>SNAMATNLIGLDTTQSQKLANALNNLLANYQVFYMNTRGYHWNIQGKEFFELHAKFEEIYTDLQLKIDELAERILTLSARPMHSFSGYLKAAQIKEHTDSIDGRSSMQGLVDGFSILLHQQRDILELAGETGDEGTSALMSDYIREQ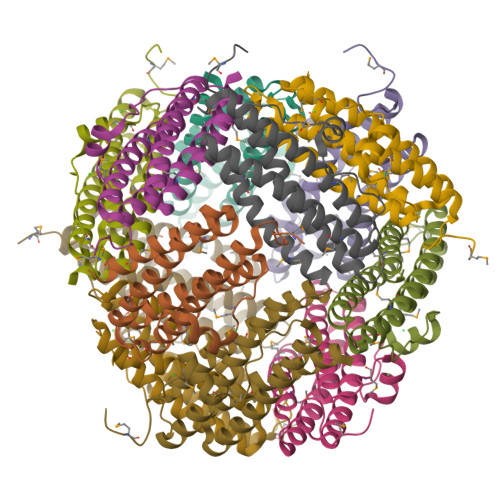EKLVWMLNAWLK[4x]>MSTNNPQTREWQNLSGEHHLAPFSDYKQLKEKGPRIITKAQGVHLWDSEGHKILDGMAGLWCVAVGYGREELVQAAEKQMRELPYYNLFFQTAHPPALELAKAITDVAPEGMTHVFFTGSGSEGNDTVLRMVRHYWALKGKPHKQTIIGRINGYHGSTFAGACLGGMSGMHEQGGLPIPGIVHIPQPYWFGEGGDMTPDAFGIWAAEQLEKKILEVGEDNVAAFIAEPIQGAGGVIIPPETYWPKVKEILAKYDILFVADEVICGFGRTGEWFGSDYYDLKPDLMTIAKGLTSGYIPMGGVIVRDKVAKVISEGGDFNHGFTYSGHPVAAAVGLENLRILRDEQIVEKARTEAAPYLQKRLRELQDHPLVGEVRGLGMLGAIELVKDKATRSRYEGKGVGMICRTFCFENGLIMRAVGDTMIIAPPLVISHAEIDELVEKARKCLDLTLEAIR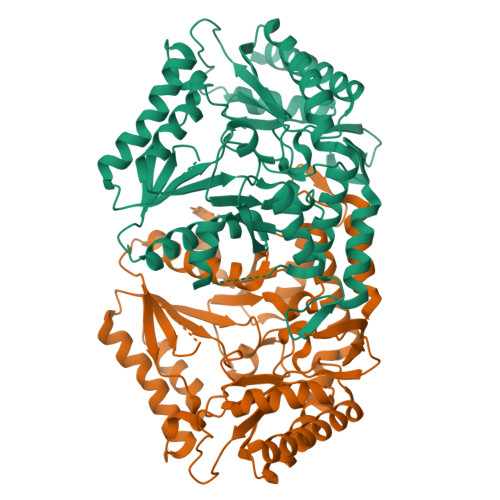LE[2x]> QVHLTHFELEGLRCLV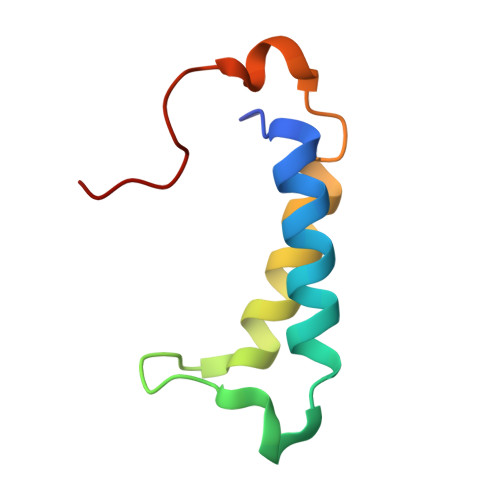DKLESLPLHKKCVPTGIEDEDALIADVKILLEELASSDPKLALTGVPIVQWP>[4x]GHAKSVPSRYSLVFDADRQVNAAAGAQPAPIKIRVLLLRSDAEFMDADFFSLQNDAKSVLGNSLLDSDQFFLTPGQTGKKLGGQSALDARYIGVIAEYQNLDGKTWRISLPLPEPTETNFYKVWQFSPDELEAHIVAGVSGLRPVKKVD

Lip is a membrane-bound lipoprotein and a core component of the type VI secretion system found in Gram-negative bacteria. Genetic studies indicate that in S. marcescens this lipoprotein (SmLip) makes an essential contribution to the basic function of the T6SS and to T6SS-dependent antibacterial killing activity. The protein fold is dominated by an eight-stranded β-sandwich and identifies SmLip as a new member of the transthyretin family of proteins. The pro­pensity to self-associate using parts of the SmLip structure that will be exposed in the periplasm suggests that this protein, exploiting the lipid anchor, helps to bind and position different components of the secretion apparatus at the outer mem­brane.

The structure of a Lip construct (residues 29–176) from Serratia marcescens (SmLip) has been determined at 1.92 Å resolution. The structure is that of the globular domain lacking only the lipoprotein signal peptide and the lipidated N-terminus of the mature protein. We now report the high-resolution structure of SmLip determined following phase determination using single-wavelength anomalous dispersion (SAD) measurements based on the scattering properties of iodide ions. The refinement proceeded with the release of NCS restraints and the incorporation of water molecules, an Na+ ion, ethylene glycol and a number of side chains with dual rotamer conformations. This data set was derived from crystals grown in the presence of chloride instead of iodide. However, we did not assign any chloride ions to the structure, noting that typical water molecules occupy the previously identified iodide-binding sites. Molecule A consists of residues 32–173; molecule B of residues 33–142 and 147–176; molecule C of residues 34–50, 53–143 and 147–175; and molecule D of residues 33–50 and 55–175. The asymmetric unit of SmLip is a tetramer with 222 symmetry, but the assembly is distinct from that previously noted for the transthyretin protein family. The accessible surface area (ASA) of the SmLip polypeptide averages out at approximately 8350 Å2; the range is from 8200 Å2 for molecule D to 8510 Å2 for molecule A. Each molecule in the asymmetric unit interacts with two of the other three and two types of protein–protein interface are formed between molecules A–B and C–D (interface I) and between molecules A–C and B–D (interface II). The type II interface covers about 6.5% of the ASA of a molecule, a level typical of the values observed simply owing to molecular packing in a crystal lattice. This interface is formed by the antiparallel alignment of two β4 strands.>[2x]PKTQRGIYHNLKESEYVASNTDVTFFFSSELYLNKFLDGYQEYRKKFNKKIERVAVTPWNMDMLADITFYSEVEKRGFHAWLKGDNATWREVHVYALRIMTKPNTL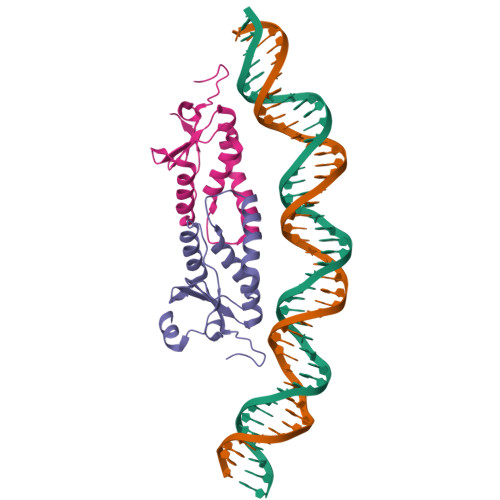DWSRIQKPRLRERRKSM> HEGVHRKPSLLAHPGPLVKSEETVILQCWSDVRFEHFLLHREGKYKDTLHLIGEHHDGVSKANFSIGPMMQDLAGTYRCYGS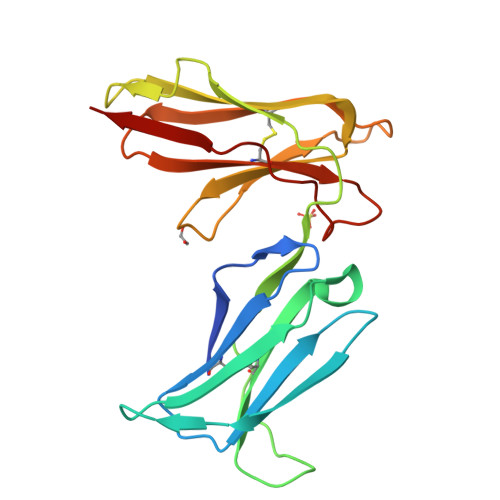VTHSPYQLSAPSDPLDIVITGLYEKPSLSAQPGPTVLAGESVTLSCSSRSSYDMYHLSREGEAHERRFSAGPKVNGTFQADFPLGPATHGGTYRCFGSFRDSPYEWSNSSDPLLVSVT>MHHHHHHTPQPTDAQPTDAQPTDLYFDFLCPYAWRGVEMAHVLRGSGEGFRLRHFSLVQGNHPQNKDQETVQWWLTDQPLGAEGGSGYMKYQRPSLNAFLAAHAAARQGEEKSWAFALALFRLHHEDKRDLDEAAFQDAATR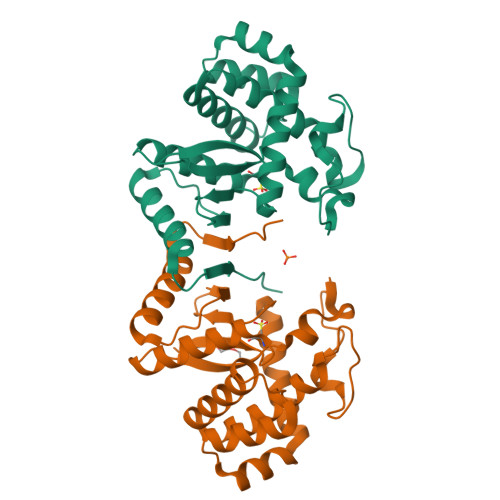AGLDLSQWKQDRQDEAGLRRELRADLEAAAALGVFGTPTFDLGGGDVAYFKFEELTRDPQAARDLWNLFTSTLRSEARVATIRRPVPKKG[2x]> PRDCQELFQVGERQSGLFEIQPQGSPPFLVNCKMTSDGGWTVIQRRHDGSVDFNRPWEAYKAGFGDPHGEFWLGLEKVHSITGDRNSRLAVQLRDWDGNAELLQFSVHLGGEDTAY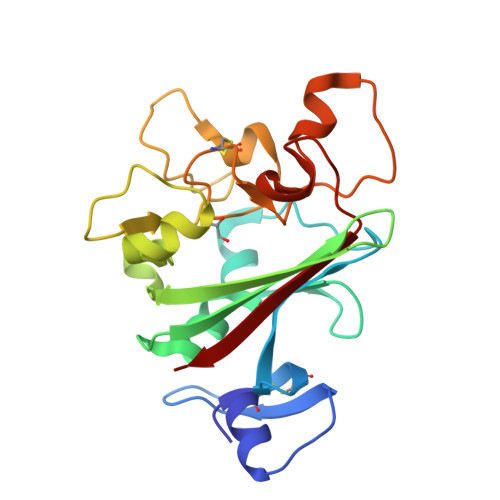SLQLTAPVAGQLGATTVPPSGLSVPFSTWDQDHDLRRDKNCAKSLSGGWWFGTCSHSNLNGQYFRSIPQQRQKLKKGIFWKTWRGRYYPLQATTMLIQPM>HMPGGSKKIGIFGGTFDPPHNGHLLMANEVLYQAGLDEIWFMPNQIPPHKQNEDYTDSFHRVEMLKLAIQSN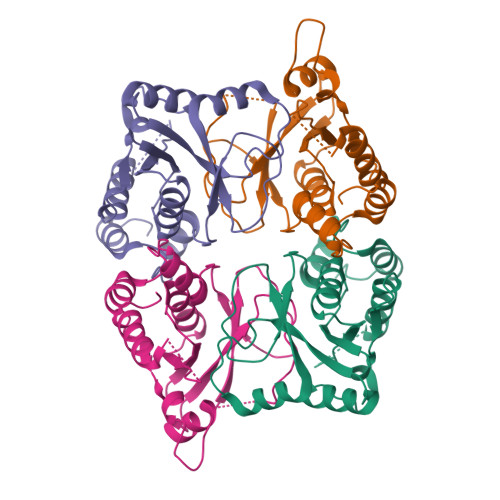PSFKLELVEMEREGPSYTFDTVSLLKQRYPNDQLFFIIGADMIEYLPKWYKLDELLNLIQFIGVKRPGFHVETPYPLLFADVPEFEVSSTMIRERFKSKKPTDYLIPDKVKKYVEENGLYES[4x]> MRKSVIAIIIIVLVVLYMSVFVVKEGERGITLRFGKVLRDDDNKPLVYEPGLHFKIPFIETVKMLDARIQTMDNQADRFVTKEKKDLIVDSYIKWRISDFSRYYLATGGGDISQAEVLLKRKFSDRLRSEIGRLD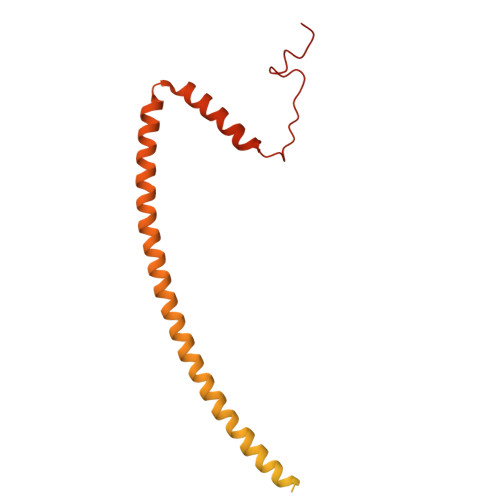VKDIVTDSRGRLTLEVRDALNSGSAGTEDEVTTPAADNAIAEAAERVTAETKGKVPVINPNSMAALGIEVVDVRIKQINLPTEVSEAIYNRMRAEREAVARRHRSQGQEEAEKLRATADYEVTRTLAEAERQGRIMRGEGDAEAAKLFADAFSKDPDFYAFIRSLRAYENSFSGNQDVMVMSPDSDFFRYMKTPTSATR>PCLNLSTNVNLDGVDTSSILSEASSTVAKIIGKPENYVMIVLKGSVPMSFGGTEDPAAYGELVSIGGLNADVNKKLSAAVSAILETKLSVPKSRFFLKFYDTKGSFFGWNGATLLEHHHHHH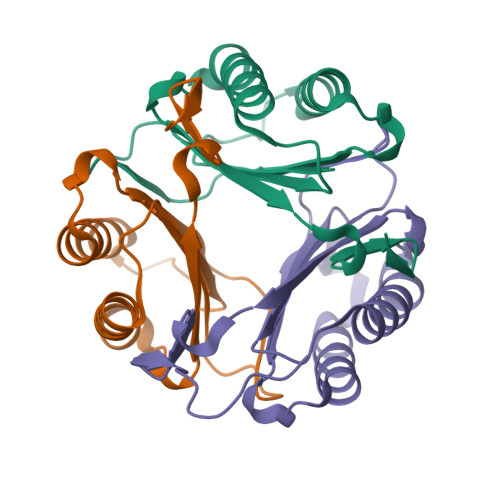[3x]> MQPAQTHAAPVRKKPSRPFVSSHHRPADDVDDGIFRVVLITSGSVASIKAPDIVGALVKSPNIDVQVVATKASTYFYSQEDVDNSVRSALNLPDGQTGEHFGVRVWTDEDEWSDWKQVGEPILHIELRRWADLVVIAPCS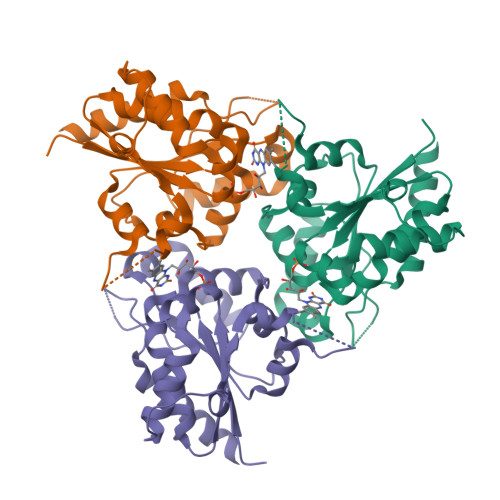ADLLAKIAGGICDSLATSLLRALGPSTPVIVCPAMNTYMYQHRLTTRHLAVVQEDLGYLVSGPQGAGRLACGDDGPGKMTDWRDIVSLIEGFATMHQDRRAVVHPGHPLQESSDPPLPPPTETPPTPGRPSKSSSAVGSSSVSTQDRAPAKAPSDDVLTGIADWRSMTNELGGDGTAWRRKWWLG AaRSs catalyze the attachment of the correct amino acid to its cognate tRNA which then is used in protein synthesis on ribosomes. Phylogenetically phenylalanyl-tRNA synthetase (PheRS), belongs to the class II aaRSs, and it is a dimer of heterodimers (αβ)2, containing two α- (PheS) and two β- (PheT) subunits. Structural studies of PheRS have shown that the α subunit binds L-Phe and ATP and is responsible for esterification catalysis. At the same time, the β subunit is involved in the recognition of the cognate tRNA molecule and editing of mis-charged tRNA.

The protein-fragment interactions were analyzed using crystal structures for five of those fragments complexed with MtPheRS/tRNAPhe (DDD00107555 (D-555), DDD01008876 (D-876), DDD00805735 (D-735), DDD00079004 (D-004) and DDD00067116 (D-116)). All five fragments occupy the L-Phe site in the α subunit of the heterotetramer. The bicyclic quinoline, quinazoline and benzimidazole moieties of the fragments are completely enclosed in the L-Phe binding site. PIEDA showed that the phenyl ring or the bicyclic core of the fragments interact with residues αPhe255 and αPhe257 through hydrophobic interaction. Residues αThr258 and αAla305 make hydrophobic interactions with the phenyl core of the fragments D-116, D-004 and D-735. In addition, a strong hydrogen bond between NH2 of D-116 and αGln215 is observed and, a proton of the protonated N of the benzoimidazole core interacts with αGlu217 through salt bridge interaction. Hydrophobic interactions with αAla305 are retained in fragments D-735, D-004 and D-116. Interestingly, 10 % DMSO increased L-Phe adenylation in the presence of the very hydrophobic D-116 fragment.

>[2x]MLSPEALTTAVDAAQQAIALADTLDVLARVKTEHLGDRSPLALARQALAVLPKEQRAEAGKRVNAARNAAQRSYDERLATLRAERDAAVLVAEGIDVTLPSTRVPAGARHPIIMLAEHVADTFIAMGWELAEGPEVETEQFNFDALNFPADHPARGEQDTFYIAPEDSRQLLRTHTSPVQIRTLLARELPVYIISIGRTFRTDELDATHTPIFHQVEGLAVDRGLSMAHLRGTLDAFARAEFGPSARTRIRPHFFPFTEPSAEVDVWFANKIGGAAWVEWGGCGMVHPNVLRATGIDPDLYSGFAFGMGLERTLQFRNGIPDMRDMVEGDVRFSLPFGVGA;>[2x]QSNAMRLPYSWLREVVAVGASGWDVTPGELEQTLLRIGHEVEEVIPLGPVDGPVTVGRVADIEELTGYKKPIRACAVDIGDRQYREIICGATNFAVGDLVVVALPGATLPGGFTISARKAYGRNSDGMICSAAELNLGADHSGILVLPPGAAEPGADGAGVLGLDDVVFHLAITPDRGYCMSVRGLARELACAYDLDFVDPASNSRVPPLPIEGPAWPLTVQPETGVRRFALRPVIGIDPAAVSPWWLQRRLLLCGIRATCPAVDVTNYVMLELGHPMHAHDRNRISGTLGVRFARSGETAVTLDGIERKLDTADVLIVDDAATAAIGGVMGAASTEVRADSTDVLLEAAIWDPAAVSRTQRRLHLPSEAARRYERTVDPAISVAALDRCARLLADIAGGEVSPTLTDWRGDPPCDDWSPPPIRMGVDVPDRIAGVAYPQGTTARRLAQIGAVVTHDGDTLTVTPPSWRPDLRQPADLVEEVLRLEGLEVIPSVLPPAPAGRGLTAGQQRRRTIGRSLALSGYVEILPTPFLPAGVFDLWGLEADDSRRMTTRVLNPLEADRPQLATTLLPALLEALVRNVSRGLVDVALFAIAQVVQPTEQTRGVGLIPVDRRPTDDEIAMLDASLPRQPQHVAAVLAGLREPRGPWGPGRPVEAADAFEAVRIIARASRVDVTLRPAQYLPWHPGRCAQVFVGESSVGHAGQLHPAVIERSGLPKGTCAVELNLDAIPCSAPLPAPRVSPYPAVFQDVSLVVAADIPAQAVADAVRAGAGDLLEDIALFDVFTGPQIGEHRKSLTFALRFRAPDRTLTEDDASAARDAAVQSAAERVGAVLRG>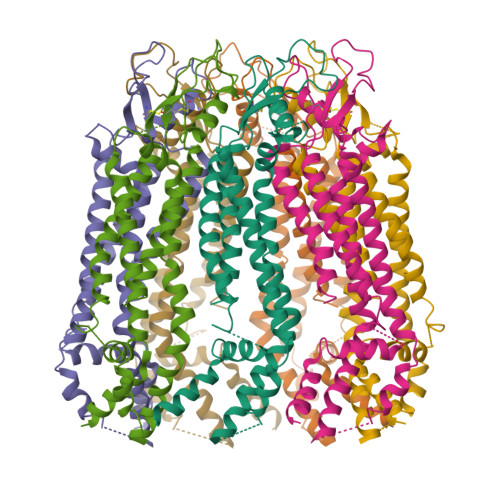[7x]MAIAQLATEYVFSDFLLKEPTEPKFKGLRLELAVDKMVTCIAVGLPLLLISLAFAQEISIGTQISCFSPSSFSWRQAAFVDSYCWAAVQQKNSLQSESGNLPLWLHKFFPYILLLFAILLYLPPLFWRFAAAPHICSDLKFIMEELDKVYNRAIKAAKSARDLDMRDGACSVPGVTENLGQSLWEVSESHFKYPIVEQYLKTKKNSNNLIIKYISCRLLTLIIILLACIYLGYYFSLSSLSDEFVCSIKSGILRNDSTVPDQFQCKLIAVGIFQLLSVINLVVYVLLAPVVVYTLFVPFRQKTDVLKVYEILPTFDVLHFKSEGYNDLSLYNLFLEENISEVKSYKCLKVLENIKSSGQGIDPMLLLTNLGMIKMDVVDGKTPMSAEMREEQGNQTAELQGMNIDSETKANNGEKNARQRLLDSSCLEWSHPQFEK> YDGTHCKAPGNCWEPKPGFPEKIAGSKY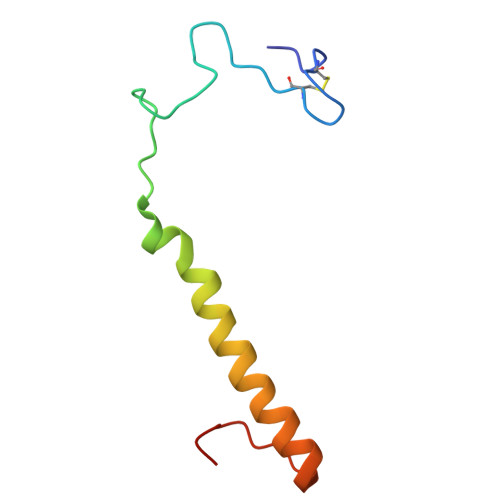DPKHDPKELNKQVESRKGEEERNANRAEHFKKTGKWVYDVKKIQ CY5.5-PEG2 | C50 H65 N3 O16 S4 | 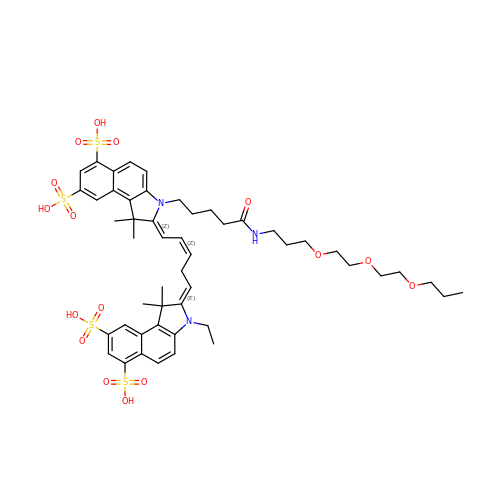ZUDVNXAIDCSDCG-HWRGAIJTSA-N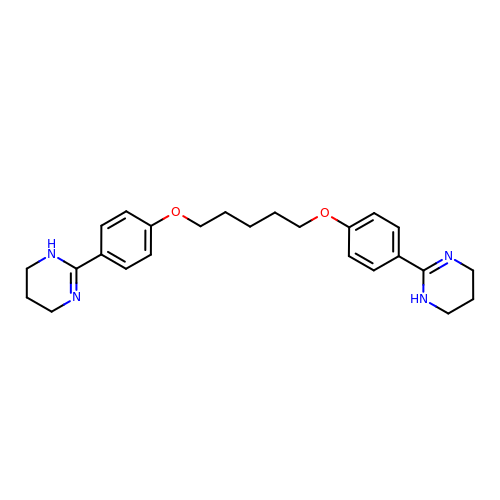2,2'-[pentane-1,5-diylbis(oxybenzene-4,1-diyl)]di-1,4,5,6-tetrahydropyrimidine | C25 H32 N4 O2 | KPYLNHFSSDNDFO-UHFFFAOYSA-N>[3x]MSVKIDVIRVEIPEGTNVIIGQSHFIKTVEDLYETLASSSPHLKFGIAFCEASGKRLIRWDGNDEELIK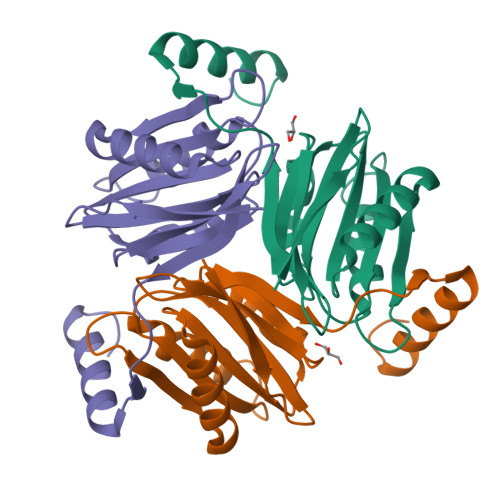LAQQTALKIGAGHTFVIYIKNGFPINVLNRIKNVEEVVRIFAATANPLQVLVAETDQGRGVIGVVDGYTPLGIETEADIKERKELLRKFGYKR> GTSTQTKAGSLTIVGTGIESIGQMTLQALSYIEAAAKVFYCVIDPATEAFILTKNKNCVDLYQYYDNGKSRLNTYTQMSELMVREVRKGLDVVGVFYGHPGVFVNPSHRALAIAKSEGYRARMLPGVSAEDCLFADLCIDPSNPGCLTYEASDFLIRDRPVSIHSHLVLFQVGCVGIADFNFTGFDNNKFGVLVDRLEQEYGAEHPVVHYIAAMMPHQ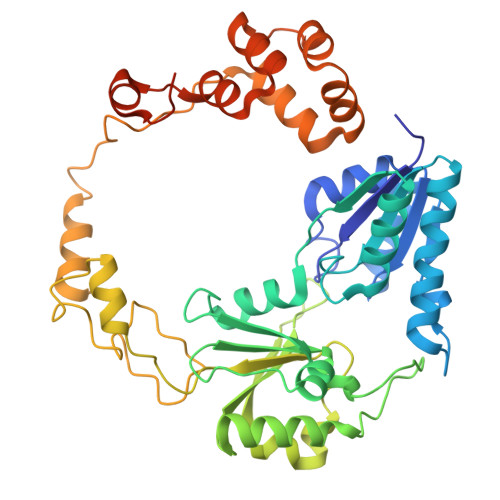DPVTDKYTVAQLREPEIAKRVGGVSTFYIPPKARKASNLDIIRRLELLPAGQVPDKKARIYPANQWEPDVPEVEPYRPSDQAAIAQLADHAPPEQYQPLATSKAMSDVMTKLALDPKALADYKADHRAFAQSVPDLTPQERAALELGDSWAIRCAMKNMPSSLLDAARESGEEASQNGFPWVIVFGVIGVIG>MACRSTLEDRSPGLASLADFPIGVAVAASGGNADIFTSSARQNIVRAEFNQITAENIMKMSYMYSGSNFSFTNSDRLVSWAAQNGQTVHGHTLVWHPSY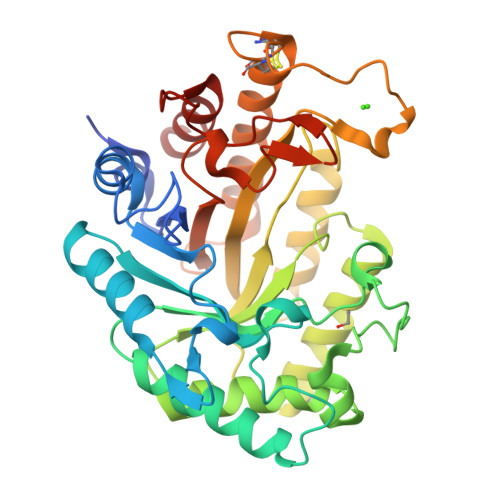QLPNWASDSNANFRQDFARHIDTVAAHFAGQVKSWDVVNEALFDSADDPDGRGSANGYRQSVFYRQFGGPEYIDEAFRRARAADPTAELYYNDFNTEENGAKTTALVNLVQRLLNNGVPIDGVGFQMHVMNDYPSIANIRQAMQKIVALSPTLKIKITELDVRLNNPYDGNSSNNYTNRNDCAVSCAGLDRQKARYKEIVQAYLEVVPPGRRGGITVWGIADPDSWLYTHQNLPDWPLLFNDNLQPKPAYQGVVEALSGR[2x]> LQLLHQKVEEQAAKYKHRVPKKCCYDGARENKYETCEQRVA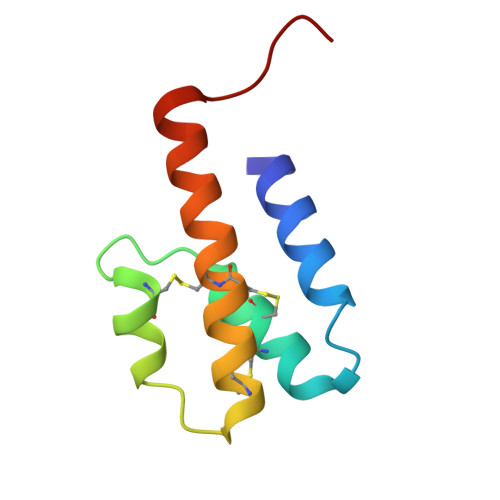RVTIGPHCIRAFNECCTIADKIRKESHHKGMLLGR>[2x]GSHMAEPQPPSGGLTDEA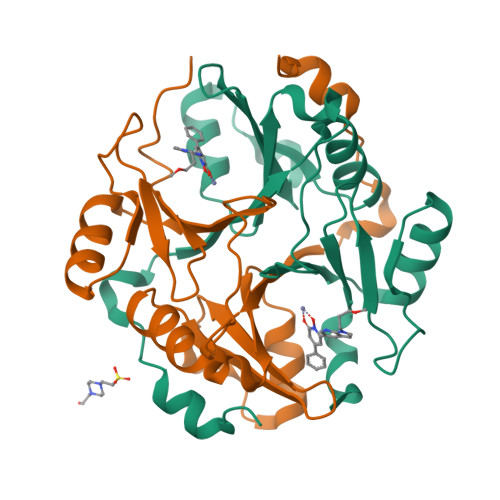ALSCCSDADPSTKDFLLQQTMLRVKDPKKSLDFYTRVLGMTLIQKCDFPIMKFSLYFLAYEDKNDIPKEKDEKIAWALSRKATLELTHNWGTEDDETQSYHNGNSDPRGFGHIGIAVPDVYSACKRFEELGVKFVKKPDDGKMKGLAFIQDPDGYWIEILNPNKMATLM>MVGGLTHVDEKGVKMVEIGYKDVVFRKAVAKGRIKLKPETVKLIKEGKIEKGNVLATAQIAGILAVKRTPELIPLC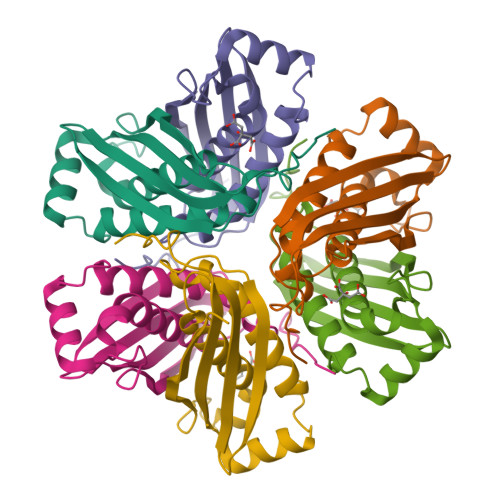HPIPITGVDITFDFGEDYIEVTCEVRAYYKTGVEMEALTGVTVALLAIWDMVKAVEKDEKGQYPYTRIENVHVVEKVKTHNSQ[3x]> GSSCTPGTTFRNRCNTCRCGSNGRSASCTLMACPP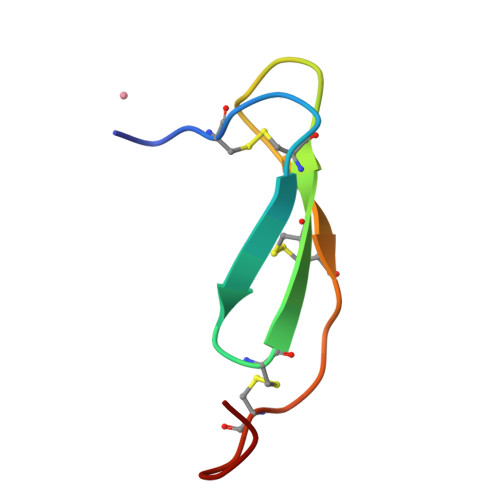GSY> MAVTATILASCGGAKTTTAEADKFDYTVEQFADLQILRYKVPEFETLTLKQKELVYYLTQAALEGRDILFDQNGKYNLRIRRMLEAVYTNYKGDKSAPDFKNMEVYLKRVWFSNGIHHHYGMEKFVPGFSQDFLKQAVLGTDAQLLPLSEGQTAEQLCDELFPVMFDPAILAKRVNQADGEDLVLTSACNYYDGVTQQEAESFYGAMKDPKDETPVSYGLNSRLVKEDGKIQEKVWKVGGLYTQAIEKIVYWLKKAETVAENDAQKAVISKLIQFYETGSLKDFDEYAILWVKDLDSRIDFVNGFTESYGDPLGVKASWESLVNFKDLDATHRTEIISSNAQWFEDHSPVDKSFKKEKVKGVSAKVITAAILAGDLYPATAIGINLPNANWIR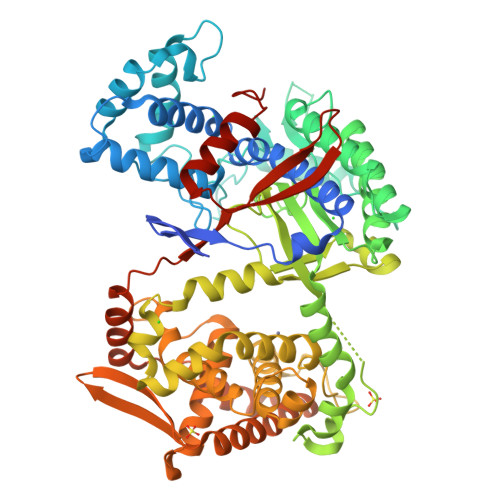AHHGSKSVTIGNITDAYNKAAHGNGFNEEFVCNDEERQRIDQYGDLTGELHTDLHECLGHGSGKLLPGVDPDALKAYGSTIEEARADLFGLYYVADPKLVELKLVPDAEAYKAEYYTFLMNGLMTQLVRIEPGNNIEEAHMRNRQLIARWVFEKGAPDKVVEMVKKDGKTYVVVNDYEKVRQLFGELLAEIQRIKSTGDFEGARTLVENYAVKVDPALHAEVLARYKKLNLAPYKGFINPVYELVTDKDGNITDVTVSYNEDYVEQMLRYSKDYSPLPSVNNLEHHHHHH(3R)-3-ethyl-1-(5-fluoropyridin-2-yl)pyrrolidin-3-ol | C11 H15 F N2 O | 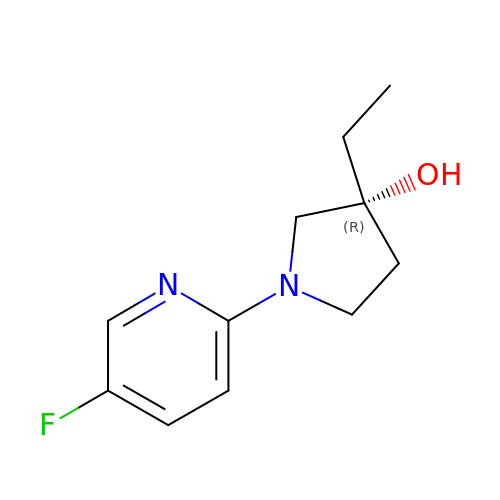OIWCZMXIAXESKW-LLVKDONJSA-N> GEIQWMRPSKEVGYPIINAPSKTKLEPSAFHYVFEGVKEPAVLTKNDPRLKTDFEEAIFSKYVSNKITEVDEYMKEAVDHYAGQLMSL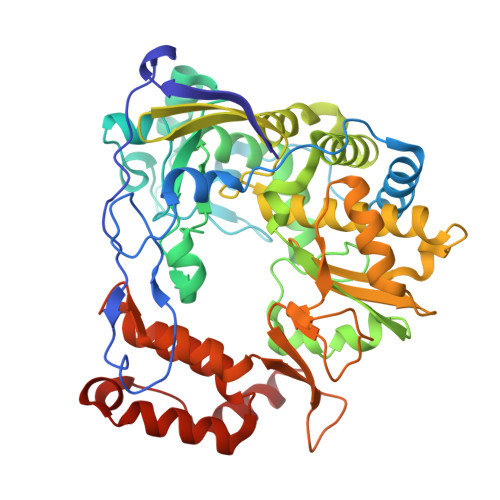DINTEQMCLEDAMYGTDGLEALDLSTSAGYPYVAMGKKKRDILNKQTRDTKEMQKLLDTYGINLPLVTYVKDELRSKTKVEQGKSRLIEASSLNDSVAMRMAFGNLYAAFHKNPGVITGSAVGCDPDLFWSKIPVLMEEKLFAFDYTGYDASLSPAWFEALKMVLEKIGFGDRVDYIDYLNHSHHLYKNKTYCVKGGMPSGCSGTSIFNSMINNLIIRTLLLKTYKGIDLDHLKMIAYGDDVIASYPHEVDASLLAQSGKDYGLTMTPADKSATFETVTWENVTFLKRFFRADEKYPFLIHPVMPMKEIHESIRWTKDPRNTQDHVRSLCLLAWHNGEEEYNKFLAKIRSVPIGRALDLPEYSTLYDRWLDSF>MNSVVNNILKAHPHQTKSFYVSSPKIVEDLIDQWTILFPRVTPHYAVKCNNDEVLLKTMCDKNVNFDCASSSEIKKVIQIGVSPSRIIFAHTMKTIDDLIFAKDQGVDIAT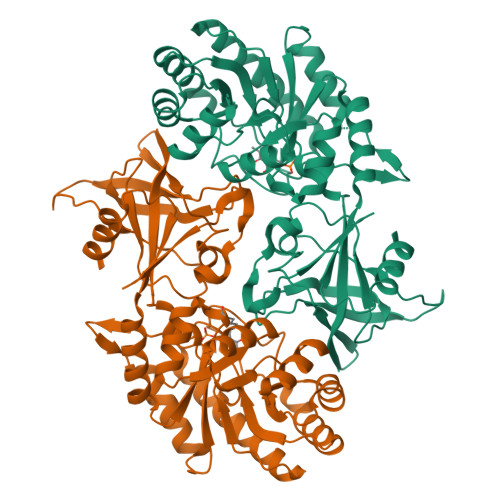FDSSFELDKIHTYHPNCKMILRIRCDDPNAAVQLGNKFGANEDEIRHLLEYAKQLDIEVIGISFHVGSGSRNPEAYYRAIKSSKEAFNEAISVGHKPYILDIGGGLHADIDEGELSTYMSDYINDAIKDFFPEDTVTIVAEPGRFFAEHYSVLATQVIGKRVRDGLYEYFFNESTYGGFSNVIFEKSVPTPQLLRDVPDDEEYVPSVLYGCTCDGVDVINHNVALPELHIGDWVYFPSWGAYTNVLTTSFNGFGEYDVYYI[8x]> MGSKCSNSGIECDSSGTCINPSNWCDGVSHCPGGEDENRCVRLYGPNFILQVYSSQRKSWHPVCQDDWNENYGRAACRDMGYKNNFYSSQGIVDDSGSTSFMKLNTSAGNVDIYKKLYHSDACSSKAVVSL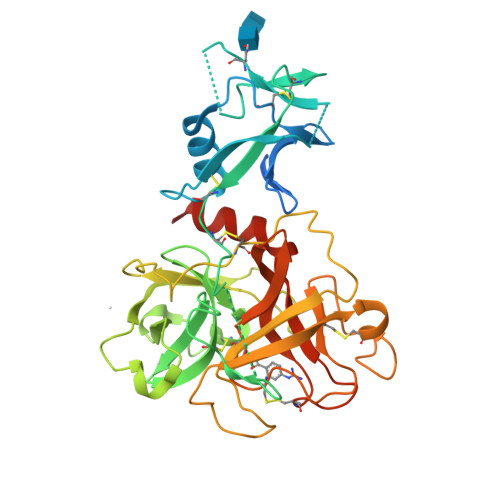RCIACGVNLNDDDDKIVGGESALPGAWPWQVSLHVQNVHVCGGSIITPEWIVTAAHCVEKPLNNPWHWTAFAGILRQSFMFYGAGYQVEKVISHPNYDSKTKNNDIALMKLQKPLTFNDLVKPVCLPNPGMMLQPEQLCWISGWGATEEKGKTSEVLNAAKVLLIETQRCNSRYVYDNLITPAMICAGFLQGNVDSCQGDSGGPLVTSKNNIWWLIGDTSWGSGCAKAYRPGVYGNVMVFTDWIYRQMRADGEFVEHHHHHHHH>[2x]MSSIKIECVLPENCRCGESPVWEEVSNSLLFVDIPAKKVCRWDSFTKQVQRVTMDAPVSSVALRQSGGYVATIGTKFCALNWKEQSAVVLATVDNDKKNNRFNDGKVDP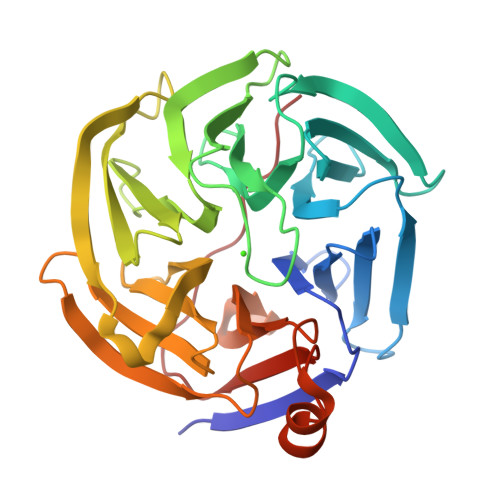AGRYFAGTMAEETAPAVLERHQGALYSLFPDHHVKKYFDQVDISNGLDWSLDHKIFYYIDSLSYSVDAFDYDLQTGQISNRRSVYKLEKEEQIPDGMCIDAEGKLWVACYNGGRVIRLDPVTGKRLQTVKLPVDKTTSCCFGGKNYSEMYVTCARDGMDPEGLLRQPEAGGIFKITGLGVKGIAPYSYAG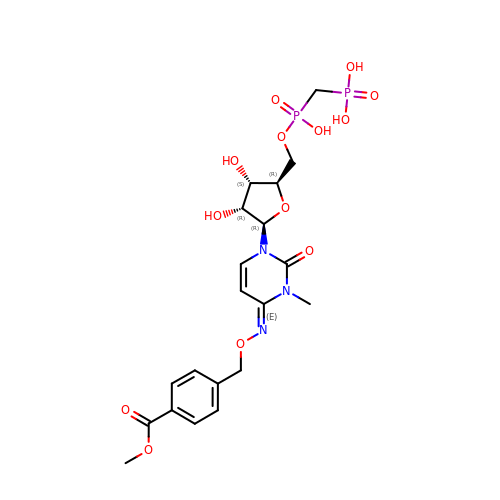[[(2~{R},3~{S},4~{R},5~{R})-5-[(4~{E})-4-[(4-methoxycarbonylphenyl)methoxyimino]-3-methyl-2-oxidanylidene-pyrimidin-1-yl]-3,4-bis(oxidanyl)oxolan-2-yl]methoxy-oxidanyl-phosphoryl]methylphosphonic acid | C20 H27 N3 O13 P2 | DUDOUSZQLIRFAY-WOXOIZPKSA-N tert-butyl {(1R,4s)-4-[(5M)-2-[(2S)-1-(3-tert-butylphenyl)-6-oxopiperidin-2-yl]-5-(3,5-dimethyl-1,2-oxazol-4-yl)-1H-benzimidazol-1-yl]cyclohexyl}carbamate 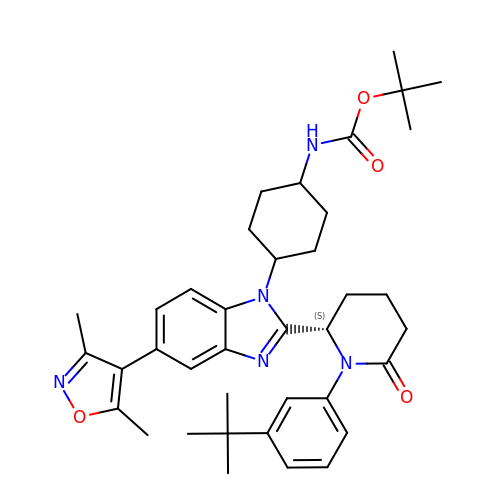| C38 H49 N5 O4 | XCKDYTZQUKRVJL-NGKQEFFVSA-N> QFAKPEDAVKYRQSALTLMASHFGRMTPV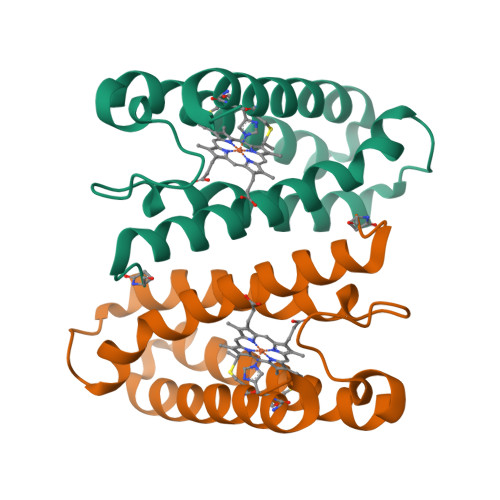VKGQAPYDAAQIKANVEVLKTLSALPWAAFGPGTEGGDARPEIWSDAASFKQKQQAFQDNIVKLSAAADAGDLDKLRAAFGDVGASCKACHDAYRKKK SigW is one of ECF sigma factors in the gram-positive model bacterium Bacillus subtilis. Its activity is suppressed by the anti-sigma RsiW under normal growth conditions. The cytoplasmic domain (RsiWcyto) interacts tightly with SigW to inhibit SigW activity. In the structure, RsiWcyto interacts with the groove formed along the surface of two domains in SigW (σW2 and σW4), resulting in the burial of the promoter binding area of SigW.

To confirm whether RsiWcyto still binds to SigW in the absence of zinc ions, SigW and RsiWcyto were co-expressed in minimal media that did not contain zinc ions and were co-purified in the absence of a reducing agent and zinc ions to oxidize the zinc coordination motif (SigW/RsiWcytoox). SigW/RsiWcytoox purified in zinc-free oxidation state was crystallized at the same condition as SigW/ RsiWcytoRed/Zn2+, and the structure was determined by molecular replacement using the structure of SigW/RsiWcytoRed/Zn2+ as a template. The final model was refined with R/Rfree values of 23.7/26.8%. Two structures of SigW/RsiWcyto in the zinc-bound and zinc-free states are superposed with an rmsd of 0.8 Å for 223 Cα atoms. This reveals that the absence of zinc ion does not change the overall conformation of SigW/RsiWcyto. The major difference between the two structures resides in the zinc-binding motif. The structure of SigW/RsiWcytoox clearly shows that a disulfide bond is formed between C3 and C37. In addition, H30 and C34 recede from the positions required for zinc coordination. Although there is a slight conformational change induced by the absence of zinc and oxidation, the interaction between SigW and RsiWcyto is not changed. In terms of the binding surface area and the number of bonds between SigW and RsiWcyto, zinc coordination of RsiW does not appear to change its ability to inhibit SigW, suggesting that SigW is not activated by oxidation or the absence of zinc in the CHCC motif of RsiW.

>MEMMIKKRIKQVKKGDQDAFADIVDIYKDKIYQLCYRMLGNVHEAEDIAQEAFIRAYVNIDSFDINRKFSTWLYRIATNLTIDRIRKKKPDYYLDAEVAGTEGLTMYSQIVADGVLPEDAVVSLELSNTIQQKILKLPDKYRTVIVLKYIDELSLIEIGEILNIPVGTVKTRIHRGREALRKQLRDL[2x];>[2x]MSCPEQIVQLMHMHLDGDILPKDEHVLNEHLETCEKCRKHFYEMEKSIALVRSTSHVEAPADFTANVMAKLPKEKKRASV>[2x]XCUCGUUUGAGCGAGUAUA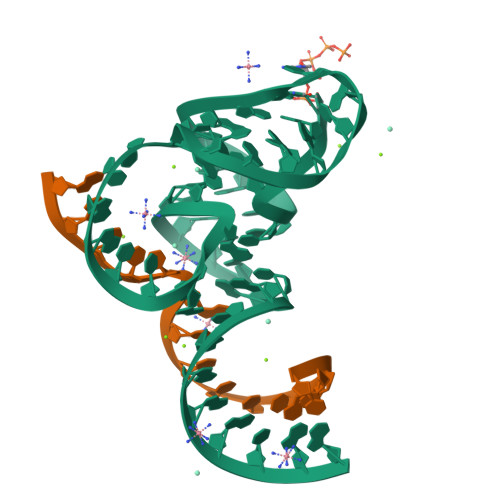AACAGUUGGUUAGGCUCAAAGCGGAGAGCAG;>UCUGCUCUCGUCCAA[2x]>TDTTLPPDDSLDRIEPVDIEQEMQRSYIDYAMSVIVGRALPEVRDGLKPVHRRVLYAMFDSGFRPDRSHAKSARSVAETMGNYHPHGDSSIYDSLVRMAQPWSLRYPLVDGQGNFGSPGNDPPAAMRYTEARLTPLAMEMLREIDEETVDFIPNYDGRVQEPTVLPSRFPNLLANGSGGIAVGMATNIPPHNLRELADAVFWALENHDADEEETLAAVMGRVKGPDFPTAGLIVGSQGTADAYKTGRGSIRMRGVVEVEEDSRGRTSLVITELPYQVNHDNFITSIAEQVRDGKLAGISNIEDQSSDRVGLRIVIEIKRDAVAKVVINNLYKHTQLQTSFGANMLAIVDGVPRTLRLDQLIRYYVDHQLDVIVRRTTYRLRKANERAHILRGLVKALDALDEVIALIRASETVDIARAGLIELLDIDEIQAQAILDMQLRRLAALERQRIIDDLAKIEAEIADLEDILAKPERQRGIVRDELAEIVDRHGDDRRTRIIAIGSG[2x];>SNALVRRKSATDIGGLPGKLADCRSTDPRKSELYVVEGDSAGGSAKSGRDSMFQAILPLRGKIINVEKARIDRVLKNTEVQAIITALGTGIHDEFDIGKLRYHKIVLMADADVDGQHISTLLLTLLFRFMRPLIENGHVFLAQPPLYKLKWQRSDPEFAYSDRERDGLLEAGLKAGKKINKEDGIQRYKGLGEM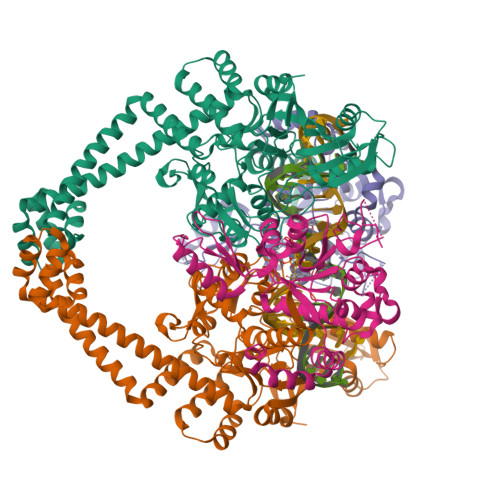DAKELWETTMDPSVRVLRQVTLDDAAAADELFSILMGEDVDARRSFITRNAKDVRFLDV[2x]>[2x]MATTTPERVMQETMDYHALNAMLNLYDKAGHIQFDKDQQAIDAFFATHVRPHSVTFASQHERLGTLVREGYYDDAVLARYDRAFVLRLFEHAHASGFRFQTFLGAWKFYTSYTLKTFDGKRYLEHFEDRVTMVALTLAQGDETLATQLTDEMLSGRFQPATPTFLNCGKQQRGELVSCFLLRIEDNMESIGRAVNSALQLSKRGGGVAFLLSNLREAGAPIKRIENQSSGVIPVMKMLEDAFSYANQLGARQGAGAVYLHAHHPDILRFLDTKRENADEKIRIKTLSLGVVIPDITFRLAKENAQMALFSPYDIQRRYGKPFGDIAISERYDELIADPHVRKTYINARDFFQTLAEIQFESGYPYIMFEDTVNRANPIAGRINMSNLCSEILQVNSASRYDDNLDYTHIGHDISCNLGSLNIAHVMDSPDIGRTVETAIRGLTAVSDMSHIRSVPSIAAGNAASHAIGLGQMNLHGYLAREGIAYGSPEALDFTNLYFYTITWHAVHTSMRLARERGKTFAGFAQSRYASGDYFTQYLQDDWQPKTAKVRALFARSGITLPTREMWLKLRDDVMRYGIYNQNLQAVPPTGSISYINHATSSIHPIVAKIEIRKEGKTGRVYYPAPFMTNENLDMYQDAYDIGPEKIIDTYAEATRHVDQGLSLTLFFPDTATTRDINKAQIYAWRKGIKSLYYIRLRQLALEGTEIEGCVSCAL;>[2x]MKLSRISAINWNKIQDDKDLEVWNRLTSNFWLPEKVPLSNDIPAWQTLSAAEQQLTIRVFTGLTLLDTIQNIAGAPSLMADAITPHEEAVLSNISFMEAVHARSYSSIFSTLCQTKEVDAAYAWSEENPPLQRKAQI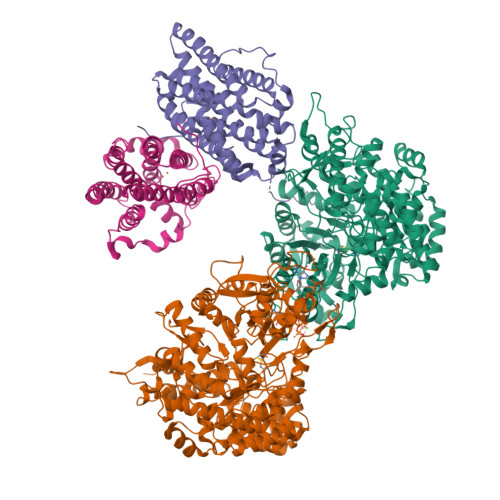ILAHYVSDEPLKKKIASVFLESFLFYSGFWLPMYFSSRGKLTNTADLIRLIIRDEAVHGYYIGYKYQIALQKLSAIEREELKLFALDLLMELYDNEIRYTEALYAETGWVNDVKAFLCYNANKALMNLGYEALFPPEMADVNPAILAALSPNADENHDFFSGSGSSYVMGKTVETEDEDWNF> MISLVFVLLIGAAFAT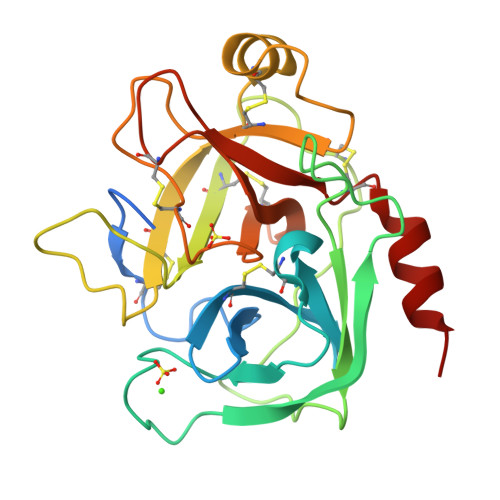EDDKIVGGYECKPYSQPHQVSLNSGYHFCGGSLVNENWVVSAAHCYKSRVEVRLGEHNIKVTEGSEQFISSSRVIRHPNYSSYNIDNDIMLIKLSKPATLNTYVQPVALPTSCAPAGTMCTVSGWGNTMSSTADSNKLQCLNIPILSYSDCNNSYPGMITNAMFCAGYLEGGKDSCQGDSGGPVVCNGELQGVVSWGYGCAEPGNPGVYAKVCIFNDWLTSTMASY> MLADTTTVNGGTIHFKGEVVNAACAVDAGSVDQTVQLGQVRTASLKQAGATSSAVGFNIQLNDCDTTVATKAAVAFLGTAIDATRTDVLALQSSAAG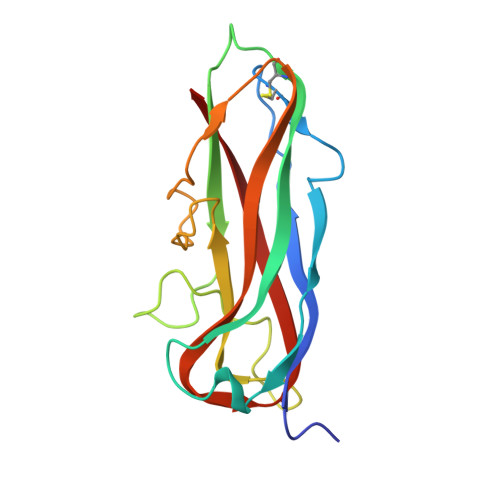SATNVGVQILDRTGNALTLDGATFSAQTTLNNGTNTIPFQARYYAIGEATPGAANADATFKVQYQ> IKSALLVLEDGTQFHGRAIGATGSAVGEVVFNTSMTGYQEILTDPSYSRQIVTLTYPHIGNVGTNDADEESSQVHAQGLVIRDLPLIASNFRNTEDLSSYLKRHNIVAIADIDTRKLTRLLREKGAQNGCIIAGDNPDAALALEKARAFPGLNGMDLAKEVTTAEAYSWTQGSWTLTGGLPQAKKEDELPFHVVAYDFGAKRNILRMLVDRGCRLTIVPAQ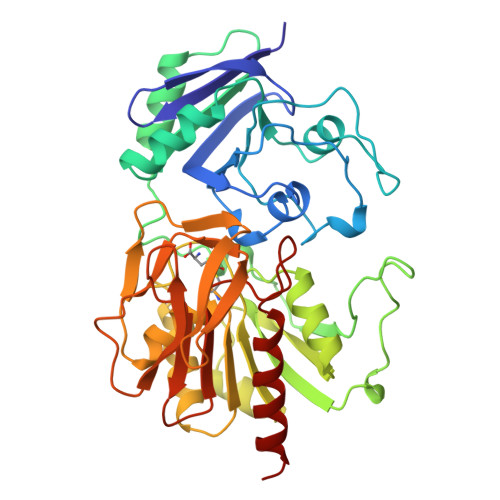TSAEDVLKMNPDGIFLSNGPGDPAPCDYAITAIQKFLETDIPVFGICLGHQLLALASGAKTVKMKFGHHGGNHPVKDVEKNVVMITAQNHGFAVDEATLPANLRVTHKSLFDGTLQGIHRTDKPAFSFQGNPEASPGPHDAAPLFDHFIELIEQYRKT> GMISPERLRVYRFFASLTDEQLKDIALISEEKSFPTGSVIFKENSKADNLMLLLEGGVELFYSNGGAGSAANSTVCSVVPGAIFGVSSLIKPYHYTSSAR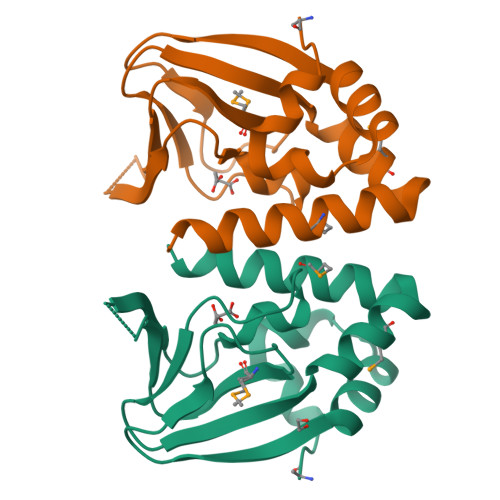ATKPVRVVDINGARLREMSENNQALGQVLMNNVAAAVLARLH> ARTKQTQDRFVY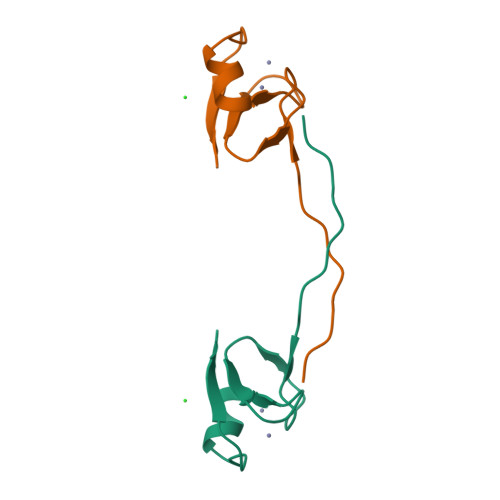TCNECKHHVETRWHCTVCEDYDLCITCYNTKNHDHKMEKLGLGLD> AAKREDLEKKQQLLRAATGKAILNGIDSINKVLEHFRRKGINQHVQNGYHGIVMNNFECEPAFYTCVEVTAGNRLFYHIVDSDEVSTKILMEFNKMNLPG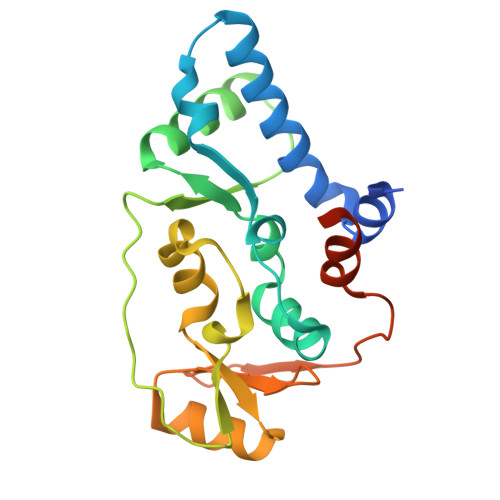EVTFLPLNKLDVRDTAYPETNDAIPMISKLRYNPRFDKAFKHVFGKTLICRSMEVSTQLARAFTMDCITLEGDQVSHRGALTGGYYDTRKSRLELQKDVRKAEEELGELEAKL1-methyl-~{N}-(1-methylcyclopropyl)-3-[(2-methyl-1,3-thiazol-5-yl)methyl]-2,4-bis(oxidanylidene)quinazoline-6-sulfonamide 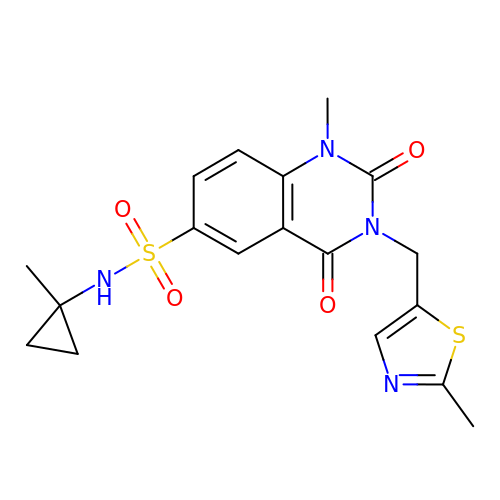| C18 H20 N4 O4 S2 | CZHJSHVWPOJSIU-UHFFFAOYSA-N>MSTNKVNKERTFLAVKPDGVARGLVGEIIARYEKKGFVLVGLKQLVPTKDLAESHYAEHKERPFFGGLVSFI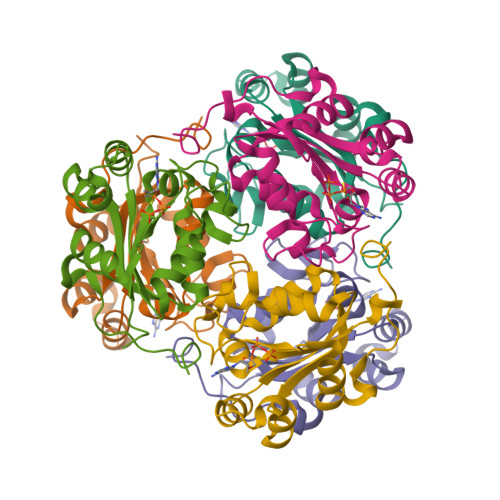TSGPVVAMVFEGKGVVASARLMIGVTNPLASAPGSIRGDFGVDVGRNIIGGSDSVESANREIALWFKPEELLTEVKPNPNLYE[6x]LL-37 is an extensively studied peptide with particular relevance in human innate immunity. LL-37 is produced as a precursor protein in human cells (e.g. leukocytes or neutrophils) and processed during its secretion to the skin, lungs, or reproductive tract. The active peptide carries a surplus of positive charge, which is attributed to interactions with the LPS or LTA of the bacterial cell wall, and negatively charged lipids of in vivo cytoplasmic membranes. We determined its atomic structure in solution and the putative membrane interaction states. Together the structures in the absence and presence of detergents revealed discrete detergent binding sites at the dimer interface indicating the presence of in vivo lipid binding sites.

We obtained two co-crystal structures, both of which are dimeric with anti-parallel helix orientations, containing two DPC (LL-37DPC-2) or six LDAO molecules (LL-37LDAO-2), respectively. The two structures superimpose with very low r.m.s.d of 0.4 Å (for 67 Cα-atoms). However, the structural deviation to LL-372 is significant (2.2 Å for 57 aligned Cα atoms) and only the core region can be reasonably aligned. NMR data using DPC micelles confirmed the detergent induced structural changes at the N-terminus of LL-37DPC-2 with a random coil rather than an α-helical structure. Furthermore, the structural disorder detected in the C-terminus of LL-37DPC-2 is in good agreement with the NMR data. When we analyzed the crystallographic environment of LL-37LDAO-2 and LL-37DPC-2 (LL-37LDAO-2 with one monomer in the AU; LL-37DPC-2 with two monomers in the AU), we noticed a ‘head-to-tail’ arrangement between the peptide dimers forming tetramers and the higher fiber-like structure oligomers. These fiber-like structures were observed in both lattice types (LL-37LDAO-2 and LL-37DPC-2) although the crystallographic environment does not correspond to each other. The ‘head-to-tail’ interfaces are formed primarily by the hydrophobic residues Phe5, Phe6 and Phe27, all of which are strongly conserved within the family of cathelicidins. These aromatic residues from adjacent chains form nest-like hydrophobic scaffold to embed two detergent molecules per nest (Phe5’, Phe6’, Phe27”, and Phe27”’) from three neighboring monomers. When we analyzed the crystallographic packing of LL-37LDAO-2 and LL-37DPC-2 in this context it turned out that one-dimensional chains are formed by hydrophobic head-to-tail interactions in both crystal forms.

>LLGDFFRKSKEKIGKEFKRIVQRIKDFLRNLVPRTES[2x]> WKIIESYEGNSYTFIDPTQLPYNEKWEFPRNNLQFGKTLGAGAFGKVVEATAFGLGKEDAVLKVAVKMLKSTAHADEKEALMSELKIMSHLGQHENIVNLLGACTHGGPVLVITEYCCYGDLLNFLRRKAEAMLGPSLAPGQDPEGLDKEDGRPLELRDLLH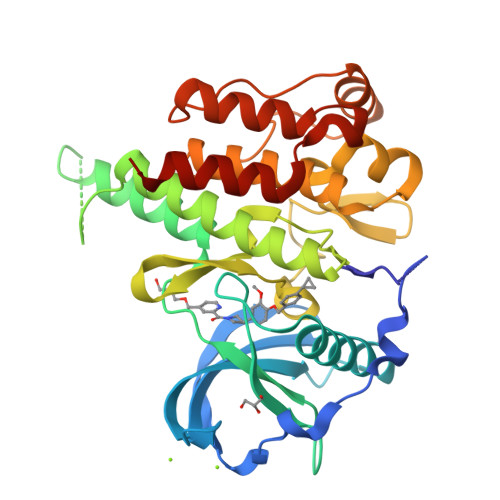FSSQVAQGMAFLASKNCIHRDVAARNVLLTNGHVAKIGDFGLARDIMNDSNYIVKGNARLPVKWMAPESIFDCVYTVQSDVWSYGILLWEIFSLGLNPYPGILVNSKFYKLVKDGYQMAQPAFAPKNIYSIMQACWALEPTHRPTFQQICSFLQEQAQEDRR> MEQQLTIEMIADAFSYDITGFDCGEEALNTFLKEHLKRQHDGQILRGYALVSGDTVPRLLGYYTLSGSCFERGML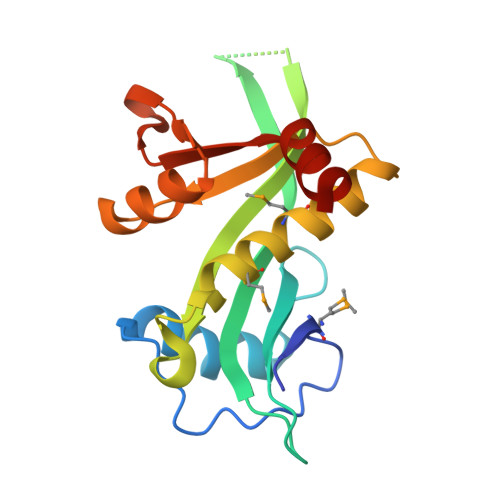PSKTQQKKIPYQNAPSVTLGRLAIDKSVQGQGWGEMLVAHVMRVVWGASKAVGIYGLFVEALNEKAKAFYLRLGFIQLVDENSNLLFYPTKSIEQLFTDDES N-(4-acetamidophenyl)-5-ethanoyl-furan-2-carboxamide | C15 H14 N2 O4 | 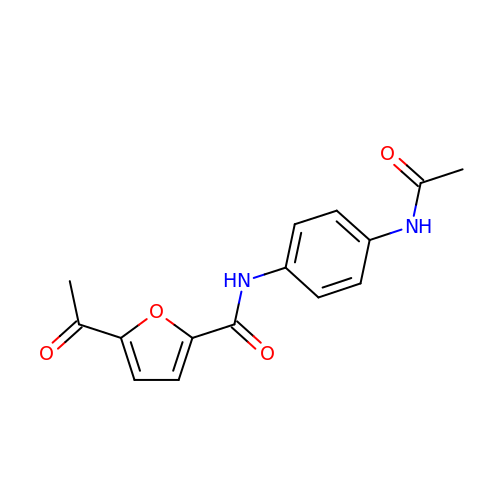VLEXAUHLNJBZLL-UHFFFAOYSA-N The core of the chitin biosynthetic machinery is an integral membrane enzyme named chitin synthase (CHS) (EC 2.4.1.16). Here we report five cryo-electron microscopy structures of a chitin synthase from the devastating soybean root rot pathogenic oomycete Phytophthora sojae (PsChs1). They represent the apo, GlcNAc-bound, nascent chitin oligomer-bound, UDP-bound (post-synthesis) and chitin synthase inhibitor nikkomycin Z-bound states of the enzyme, providing detailed views into the multiple steps of chitin biosynthesis and its competitive inhibition. The structures reveal the chitin synthesis reaction chamber that has the substrate-binding site, the catalytic centre and the entrance to the polymer-translocating channel that allows the product polymer to be discharged.

The structure of dimeric PsChs1 bound with a pre-translocating (GlcNAc)3 and a UDP in each PsChs1 protomer was obtained. This reflects the post-glycosyl transfer state during chitin biosynthesis. (GlcNAc)3 is trapped within the chitin-translocating channel through a series of interactions, including hydrogen bonds and hydrophobic interactions. The second GlcNAc moiety resides at the entrance of the channel, sandwiched between Pro454 and Trp539. The newly added GlcNAc moiety extends outside the channel, representing a pre-translocation state. As in the substrate-bound PsChs1, the uridine moiety of UDP is fixed in the uridine-binding tub. Unlike the apo structure, however, an approximately 7 Å retraction of the VLPGA loop (452–458) and an approximately 100° flip of the side chain of Pro454 are observed in the UDP/(GlcNAc)3-bound structure. As a result, the entrance of the chitin-translocating channel is opened. In the UDP/(GlcNAc)3-bound structure, the Mn2+ ion forms coordinate bonds with the β-phosphate group of the leaving group UDP with a bond length of 2.2–2.3 Å, which is consistent with the range of coordinate bonds between a first transition metal and a nitrogen-containing or oxygen-containing compound. Our PsChs1 structures revealed that the entrance to this channel is blocked by the swinging loop, specifically residue Pro454, in the apo and substrate-bound states, but it is open in the (GlcNAc)3-bound state.

>MSGAPPPSSGFAPRSYGQQPLSHAPRSSMMSVEYDGIPLPPPSIRSCGSQQYVTSYIPTGAAFPPSSVQDMISSMKSYASATDLVRTYSEIPSVEEALSTLDRAAAALNARRYRDALKLYLEGGYAMANVAERQANPKICNLLTSKGFETLNWCARLCDWIEGRIKEKHPRPGVHKVGIPVSNWDEDWVGPFMDEEEARRMWYTPVYCPHPIDFSNLGYRLRCVETGRRPRLMICITMYNEGPQQLKATLKKLANNLAYLKEQMPGDEKSLTGAFAGDDVWQNVLVCIVADGREQVHPKTLDYLEAIGLYDEDLLTINSAGIGAQCHLFEHTLQLSVNGKCLLPIQTVFALKENKASKLDSHHWYFNAFAEQIQPEYTAVMDVGTMLTKSALYHLLFAFERNHQIGGACGQLTVDNPFENLSNWVISAQHFEYKISNILDKSLESCFGFISVLPGAFSAYRYEAIRGAPLDAYFQTLNIELDVLGPFIGNMYLAEDRILSFEVVARKNCNWTMHYVKDAVARTDVPHDLVGLISQRKRWLNGAFFATLFSIWNWGRIYSESKHTFVRKMAFLVFYVYHLLYTAFGFFLPANLYLALFFIVFQGFQQNRLEFIDTSEYSQTVLDCAVYIYNFSYLFGLLMLIIIGLGNNPKHMKLTYYFVGAVFGLMMMLSSLVGAGIFFSTPATVHSIVVSILTVGVYFIASALHGEVHHIFMTFTHYTALIPSFVNIFTIYSFCNLQDLSWGTKGLHDDPLLAASLDETEKGDFKDVIAKRRALEELRREEKERVENRKKNFEAFRTNVLLTWAFSNLIFALFVVYFASSSTYMPVLYIFVASLNTCRLLGSIGHWVYIHTEGLRGRVIDKSECGNGTGRYPQNSYVQLEEHYAALAEDQRTYASGRTNASVRTVNDVSSAA[2x]> 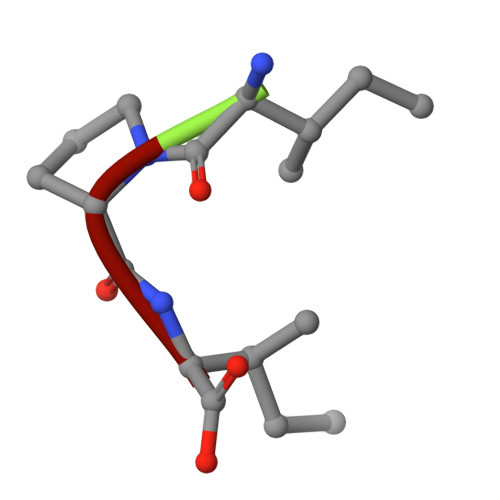IPI> MSYTPGQPVTAVVQRVEIHKLRQGENLILGFSIGGGIDQDPSQNPFSEDKTDKGIYVTRVSEGG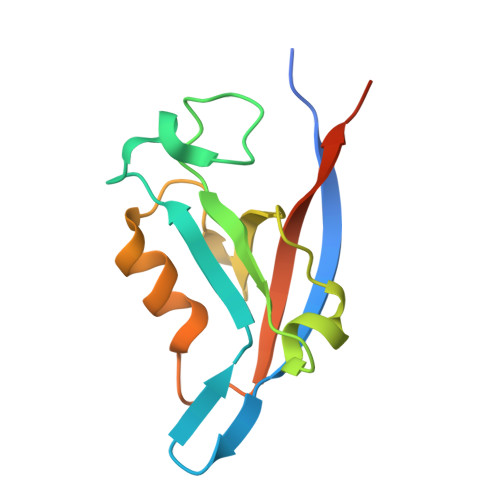PAEIAGLQIGDKIMQVNGWDMTMVTHDQARKRLTKRSEEVVRLLVTRQSLQKAVQQSMLS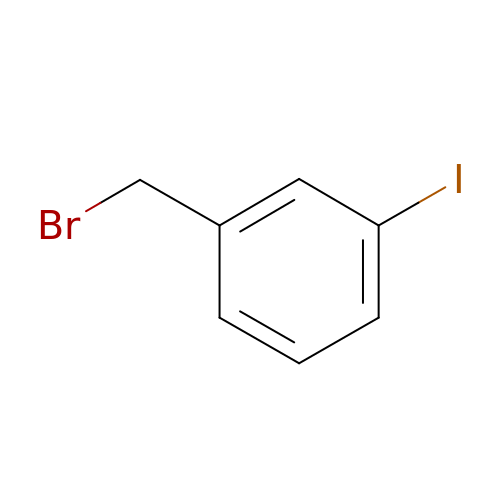Alpha-Bromo-3-Iodotoluene | C7 H6 Br I | BACZSVQZBSCWIG-UHFFFAOYSA-N> MVELTEIKDDVVQLDEPQFSRNQAIVEEKASATNNDVVDDEDDSDSDFEDEFDENETLLDRIVALKDIVPPGKRQTISNFFGFTSSFVRNAFT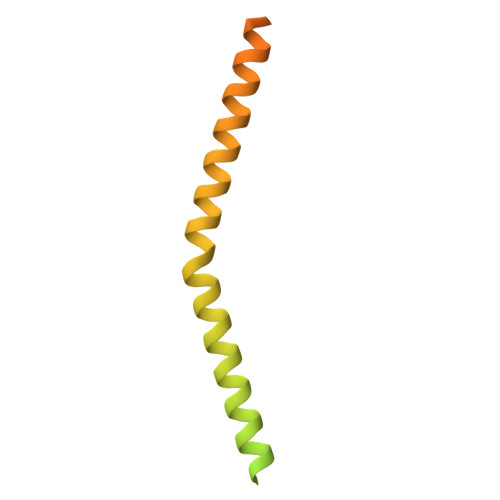KSGNLAWTLTTTALLLGVPLSLSILAEQQLIEMEKTFDLQSDANNILAQGEKDAAATANRTLQVDGSPGHHHHHHHHHH>DLILPFYKAGKVSFYQGDLDVLINFLEPDVLVNAANGDLRHVGGVARAIDVFTGGKLTKRSKE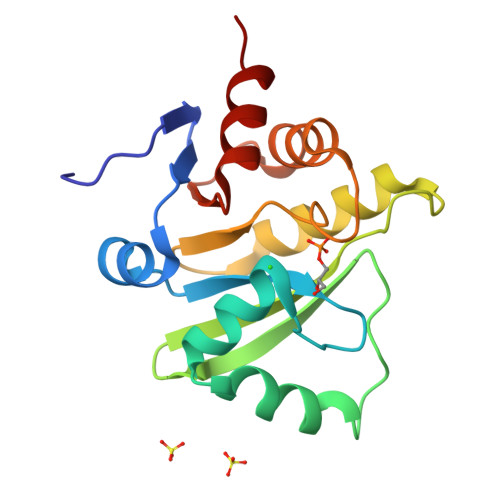YLKSSKAIAPGNAVLFENVLEHLSVLNAVGPRNGDSRVEGKLCNVYKAIAKCDGKILTPLISVGIFKVKLEVSLQCLLKTVTDRDLNVFVYTDQERVTIENFFNG[3x]{4-METHYL-3-[(1-METHYLETHYL)(2-{[3-(METHYLSULFONYL)-5-MORPHOLIN-4-YLPHENYL]AMINO}PYRIMIDIN-4-YL)AMINO]PHENYL}METHANOL 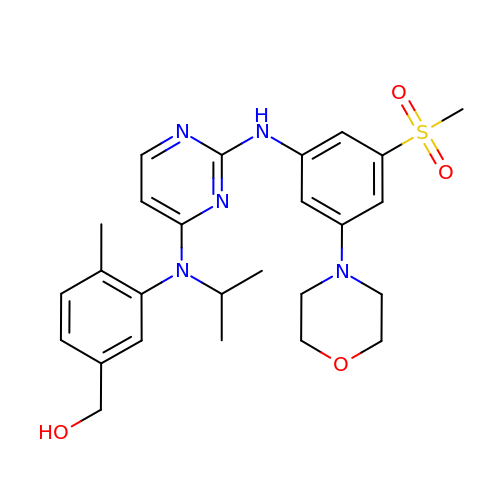| C26 H33 N5 O4 S | AAXNCGQOXAXDOW-UHFFFAOYSA-N> RYKKKWAATEPKFPAVRLALQNFDMTYSVQFGDLWPSIRVSLLSEQKYGALVNNFAAWDHVSAKLEQLSAKDFVNEAISHWELQSEGGQSAAPSPASWACSPNLRCFTFDRGDISRFPPARPGSLGVMEYYLMDAASLLPVLALGLQPGDIVLDLCAAPGGKTLALLQTGCCRNLAANDLSPSRIARLQKILHSYVPEEIRDGNQVRVTSWDGRKWGELEGDTYDRVLVDVPCTTDRHSLHEEENNIFKRSRKKERQILPVLQVQLLAAGLL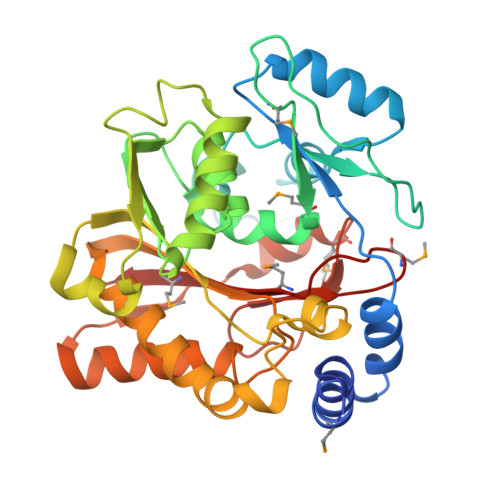ATKPGGHVVYSTCSLSHLQNEYVVQGAIELLANQYSIQVQVEDLTHFRRVFMDTFCFFSSCQVGELVIPNLMANFGPMYFCKMRRLT> MTVKSQQQIIDSFKQANQDQLFQYYDSLTIDQQQEFIDQLSTIEEPAKLISTVEQAIQFSQTNSTSRNFTQLPNEQTASTLDLSKDILQNWTELGLKAIGNGEVAVLLMAGGQGTRLGSSAPKGCFNIELPSQKSLFQIQAEKILKIEQLAQQYLKSTKKPIINWYIMTSGPTRNATESFFIENNYFGLNSHQVIFFNQGTLPCFNLQGNKI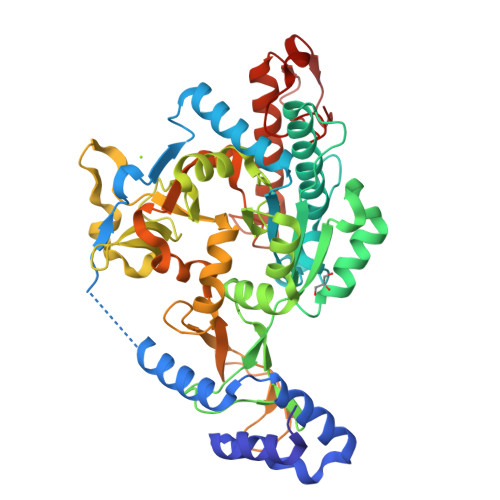LLELKNSICQSPDGNGGLYKALKDNGILDDLNSKGIKHIHMYCVDNCLVKVADPIFIGFAIAKKFDLATKVVRKRDANESVGLIVLDQDNQKPCVIEYSEISQELANKKDPQDSSKLFLRAANIVNHYYSVEFLNKMIPKWISSQKYLPFHIAKKKIPSLNLENGEFYKPTEPNGIKLEQFIFDVFPSVELNKFGCLEVDRLDEFSPLKNADGAKNDTPTTCRNHYLERSSKWVIQNGGVIDNQGLVEVDSKTSYGGEGLEFVNGKHFKNGDII>MKTIIINGVQFNTDEDTTILKFARDNNIDISALCFLNNCNNDINKCEICTVEVEGTGLVTACDTLIEDGMIINTNSDAVNEKIKSRISQLLDIHEFKCGPCNRRENCEFLKLVIKYKARASKPFLPKDKTEYVDERSKSLTVDRTKCLLCGRCVNACGKNTETYAMKFLNKNGKTIIGAEDEKCFDDTNCLLCGQCIIACPVAALSEKSHMDRVKNALNAPEKHVIVAMAPSVRASIGELFNMGFGVDVTGKIYTALRQLGFDKIFDINFGADMTIMEEATELVQRIENNGPFPMFTSCCPGWVRQAENYYPELLNNLSSAKSPQQIFGTASKTYYPSISGLDPKNVFTVTVMPCTSKKFEADRPQMEKDGLRDIDAVITTRELAKMIKDAKIPFAKLEDSEADPAMGEYSGAGAIFGATGGVMEAALRSAKDFAENAELEDIEYKQVRGLNGIKEAEVEINNNKYNVAVINGASNLFKFMKSGMINEKQYHFIEVMACHGGCVNGGGQPHVNPKDLEKVDIKKVRASVLYNQDEHLSKRKSHENTALVKMYQNYFGKPGEGRAHEILHFKYKKSAWSHPQFEK[2x]

pmcHydrogenases are metalloenzymes that catalyze the interconversion between protons (H+), electrons (e−) and hydrogen (H2). Among them, [FeFe]‐hydrogenases exhibit the highest activity for both H2 production and oxidation. Their catalytic cofactor, termed H‐cluster, consists of a [4Fe4S] sub‐cluster ([4Fe]H) and a diiron moiety ([2Fe]H) bridged through a cysteine residue. The amine base is connected to the protein surface through a conserved proton transfer pathway (PTP) for rapid H+ shuttling.

Two crystals of 1.39 Å and 1.5 Å, termed CpI‐CN−‐1 and CpI‐CN−‐2 in the following, were analyzed in depth. They were compared to two structures of CO‐treated CpI for which we obtained higher resolutions (1.34 Å and 1.52 Å; termed Hox‐CO‐1 and Hox‐CO‐2 hereafter) than previously reported. The four newly obtained structures feature strong electron densities at the OCS at Fed that are not present in the structure of untreated CpI. The refined occupancies indicate that the OCS is fully occupied by an extrinsic ligand in CN−‐treated CpI, whereas only 71 to 93 % of the OCS of CO‐treated crystals hold an extrinsic ligand. The latter is possibly due to an insufficient partial pressure of CO in the crystallization wells. CO binds to the OCS of the H‐cluster, and CO and CN− are isoelectronic, making it challenging to distinguish them by electron density analysis. To the best of our knowledge, conformational changes of PTP residues have never been observed in structures of untreated CpI wild type proteins. They are also absent from three independently prepared structures obtained by CO treatment as well as from the sulfide (SH−) ‐bound Desulfovibrio desulfuricans [FeFe]‐hydrogenase.CARBOXYMETHYLDETHIA COENZYME *A | C23 H38 N7 O18 P3 | 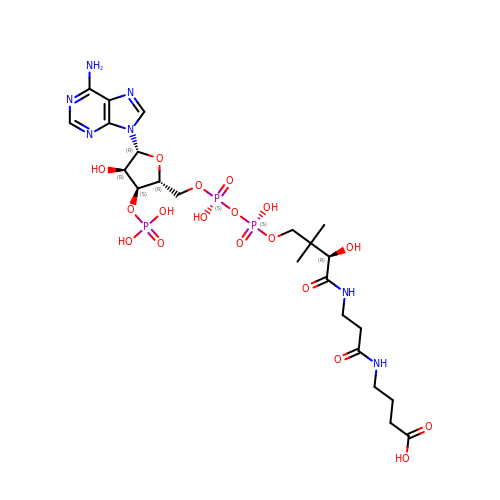SKRDARVCOPFVCP-GRFIIANRSA-N Tristromaviruses, which build enveloped filamentous virions and infect hyperthermophilic neutrophiles of the order Thermoproteales, represent one such enigmatic virus families. A cryo-electron microscopic reconstruction of the tristromavirus Pyrobaculum filamentous virus 2 at 3.4 Å resolution shows that the virion is constructed from two paralogous major capsid proteins (MCP) which transform the linear dsDNA genome of the virus into A-form by tightly wrapping around it. Unexpectedly, the two MCP are homologous to the capsid proteins of other filamentous archaeal viruses, uncovering a deep evolutionary relationship within the archaeal virosphere. Our results uncover an evolutionary relationship among three families of hyperthermophilic archaeal viruses, Tristromaviridae, Rudiviridae and Lipothrixviridae, including the homology of the MCPs and the similar compaction of the genomes as A-form DNA by these MCPs.

To study the virion organization of tristromaviruses, we have determined the structure of the Pyrobaculum filamentous virus 2 (PFV2) at 3.4 Å resolution. Cryo-electron micrographs show the membrane-enveloped virions of PFV2 to be ∼340 Å in diameter and ∼5,000 Å in length. The helical symmetry was determined to be a rise of 2.86 Å and a rotation of 22.95° per asymmetric unit, where the asymmetric unit contained a protein heterodimer and 12 bp (base pairs) of A-form DNA. The DNA, almost completely covered by the heterodimers, tightly supercoils in a solenoidal fashion with one right-handed supercoil per 45.4 Å turn of the capsid helix. The native twist of the DNA is therefore 11.3 bp/turn (564 bp in forty-seven local turns plus three supercoil turns). There was no ambiguity in fitting the sequences of MCP1 and MCP2 into the density map given the resolution achieved. While a 3D superposition of MCP1 and MCP2 shows significant differences in the overall folds, a flexible secondary structure alignment reveals a one-to-one mapping of local secondary structure elements indicative of obvious homology. Notably, PFV2 achieves a similar coverage of A-DNA as SIRV2 and AFV1 by swapping the upper half of the MCP1 N-terminal helix-arm to the other side of the MCP2 helix-arm. In contrast, this spacing is ∼30 Å in PFV2 suggesting that the lipids are arranged in a similar manner as in the host membrane, perhaps stabilized by VP3. Due to the shared virion organization, we suggest unifying Tristromaviridae and the order Ligamenvirales within a class ‘Tokiviricetes’ (toki means ‘thread’ in Georgian and viricetes is an official suffix for a virus class), the first class-rank taxon for archaeal viruses.

>MSVVTTRARIAETLTEKHTLGIEKVVATDSWRVGITSREKKLERINISAEISRRIQDEAIAYARNKGIPYLPGINGIAWKLLRLKWLGYTDQINVVMRTVPAEWRDFLTQIMENTQMESMYSELRKVRV[23x];>[23x]MSVEVYRQKIEKGGYSAAYEATRRYEREEIEVLSWSSRWESAWSKFGEAVKALGKIEGAPRALVIAKVQEALAYMSKPLPNMKLAMAAAVQAVRACEQLPGMNRERCLDAVAGALGVAKDWIRREMTGGGGGGGGGGGGGGGAVV Polythiazide | C11 H13 Cl F3 N3 O4 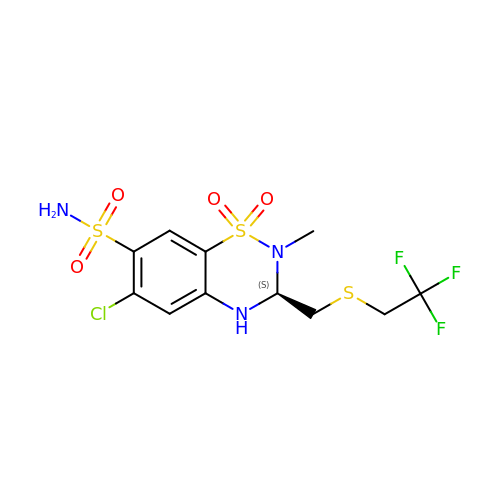S3 | CYLWJCABXYDINA-JTQLQIEISA-N>[3x]MRDTMEILRTENIVKYFGEFKALDGVSISVCKGDVTLIIGPNGSGKSTLINVITGFLKADEGRVYFENKDITNKEPAELYHYGIVRTFQTPQPLKEMTVLENLLIGEINPGESPLNSLFYKKWIPKEEEMVEKAFKILEFLKLSHLYDRKAGELSGGQMKLVEIGRALMTNPKMIVMDEP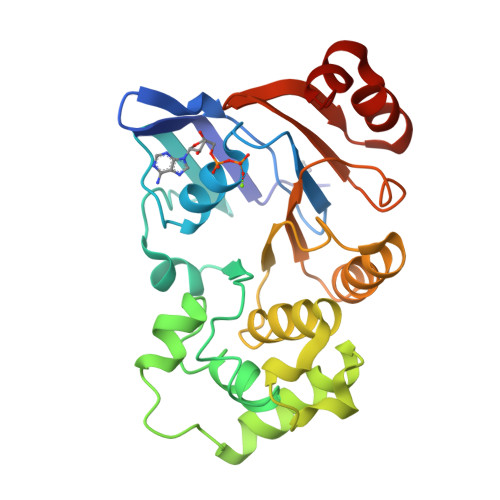IAGVAPGLAHDIFNHVLELKAKGITFLIIEHRLDIVLNYIDHLYVMFNGQIIAEGRGEEEIKNVLSDPKVVEIYIGE>MAKSGGCGAGAGVGGGNGALTWVTLFDQNNAAKKEESETANKNDSSKKLSVERVYQKKTQLEHILLRPDTYIGSVEPLTQFMWVYDEDVGMNCREVTFVPGLYKIFDEILVNAADNKQRDKNMTCIKVSIDPESNIISIWNNGKGIPVVEHKVEKVYVPALIFGQLLTSSNYDDDEKKVTGGRNGYGAKLCNIFSTKFTVETACKEYKHSFKQTWMNNMMKTSEAKIKHFDGEDYTCITFQPDLSKFKMEKLDKDIVALMTRRAYDLAGSCRGVKVMFNGKKLPVNGFRSYVDLYVKDKLDETGVALKVIHELANERWDVCLTLSEKGFQQISFVNSIATTKGGRHVDYVVDQVVGKLIEVVKKKNKAGVSVKPFQVKNHIWVFINCLIENPTFDSQTKENMTLQPKSFGSKCQLSEKFFKAASNCGIVESILNWVKFKAQTQLNKKCSSVKYSKIKGIPKLDDANDAGGKHSLECTLILTEGDSAKSLAVSGLGVIGRDRYGVFPLRGKILNVREASHKQIMENAEINNIIKIVGLQYKKSYDDAESLKTLRYGKIMIMTDQDQDGSHIKGLLINFIHHNWPSLLKHGFLEEFITPIVKASKNKQELSFYSIPEFDEWKKHIENQKAWKIKYYKGLGTSTAKEAKEYFADMERHRILFRYAGPEDDAAITLAFSKKKIDDRKEWLTNFMEDRRQRRLHGLPEQFLYGTATKHLTYNDFINKELILFSNSDNERSIPSLVDGFKPGQRKVLFTCFKRNDKREVKVAQLAGSVAEMSAYHHGEQALMMTIVNLAQNFVGSNNINLLQPIGQFGTRLHGGKDAASPRYIFTMLSTLARLLFPAVDDNLLKFLYDDNQRVEPEWYIPIIPMVLINGAEGIGTGWACKLPNYDAREIVNNVRRMLDGLDPHPMLPNYKNFKGTIQELGQNQYAVSGEIFVVDRNTVEITELPVRTWTQVYKEQVLEPMLNGTDKTPALISDYKEYHTDTTVKFVVKMTEEKLAQAEAAGLHKVFKLQTTLTCNSMVLFDHMGCLKKYETVQDILKEFFDLRLSYYGLRKEWLVGMLGAESTKLNNQARFILEKIQGKITIENRSKKDLIQMLVQRGYESDPVKAWKEAQEKAAEEDETQNQHDDSSSDSGTPSGPDFNYILNMSLWSLTKEKVEELIKQRDAKGREVNDLKRKSPSDLWKEDLAAFVEELDKVESQEREDVLAGMSGKAIKGKVGKPKVKKLQLEETMPSPYGRRIIPEITAMKADASKKLLKKKKGDLDTAAVKVEFDEEFSGAPVEGAGEEALTPSVPINKGPKPKREKKEPGTRVRKTPTSSGKPSAKKVKKRNPWSDDESKSESDLEETEPVVIPRDSLLRRAAAERPKYTFDFSEEEDDDADDDDDDNNDLEELKVKASPITNDGEDEFVPSDGLDKDEYTFSPGKSKATPEKSLHDKKSQDFGNLFSFPSYSQKSEDDSAKFDSNEEDSASVFSPSFGLKQTDKVPSKTVAAKKGKPSSDTVPKPKRAPKQKKVVEAVNSDSDSEFGIPKKTTTPKGKGRGAKKRKASGSENEGDYNPGRKTSKTTSKKPKKTSFDQDSDVDIFPSDFPTEPPSLPRTGRARKEVKYFAESDEEEDDVDFAMFN[2x]

Human TOP2 proteins, including the two isomers TOP2A and TOP2B, resolve topological stresses during DNA metabolisms such as replication, transcription, and chromosomal compaction. TOP2 catalyzes both positive and negative supercoiling as well as decatenation. TOP2A and TOP2B share 67% identity at the protein level, which is largely distinctive in the C-terminal domain (CTD). Taken together, this study suggests that activated ERK2 phosphorylates TOP2B to regulate TOP2-DNA interactions and favor transcriptional activation in IEGs.

The resultant EGR1 fragment (EGR1 #3-3, 50 bp, –30 to +20 of the TSS) was used to form TOP2B-EGR1 TSS complex. Although the protein-DNA complex itself was unstable, it could be stabilized by the addition of etoposide, a small chemical inhibitor that traps TOP2 in the TOP2-DNA cleavage complex, which is otherwise a transient intermediate. The cryo-EM structure of the ternary complex was determined at a nominal resolution of 3.9 Å. The structure contained a pseudo-symmetrical dimer of two TOP2B molecules. Although the density of the ATPase domain of TOP2B (1–456 aa) was observed in the 2D and 3D reconstructions, interpretable maps were not obtained in the 3D refinement probably because of its intrinsic flexibility relative to the core domain. Consequently, the flexible CTD (1208–1626 aa) containing ERK-phosphorylated residues was not visible. Therefore, the final model of TOP2B includes the DNA-binding and catalytic core domains (regions of 457–1118 aa and 1140–1207 aa, respectively). We observed a DNA segment docked to the central cleft of the TOP2B dimer. Both of the two DNA strands were cleaved at the active site of each TOP2B, and the DNA is bent by approximately 90°. Two etoposide molecules were intercalated into the two cleavage sites of the double strand of the EGR1 TSS.>GPLGSETKENRWVPVTVLPGCVGCRTVAALASWTVRDVKERIFAETGFPVSEQRLWRGGRELSDWIKIGDLTSKNCHLFVNLQSKG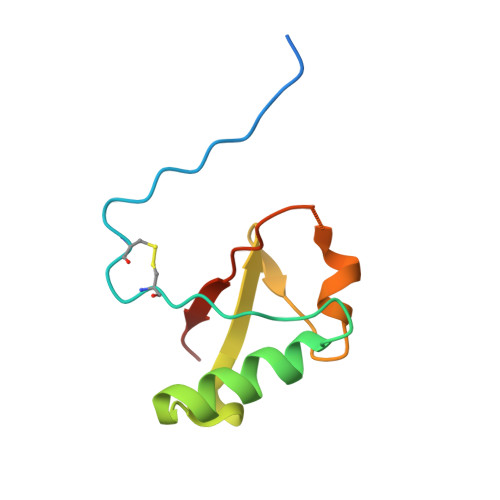LKG[2x]> MAYIAVPAVVDSRSSEAIGLLESFGVDAGADANDVSYQDHDYVLDQLQYMLDGYEAGDVIDALVHKNWLHHSVYCLLPPKSQLLEYWKSNPSAIPDNVDRRLRKRLMLKKDLRKD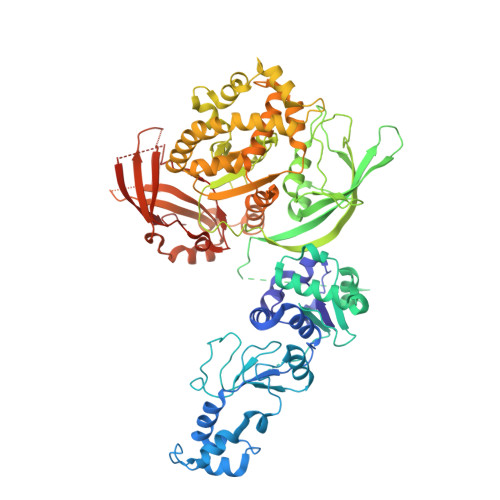DEYNQLARAFKISDVYAPLISSTTSPMTMIQNLNQGEIVYTTTDRVIGARILLYAPRKYYASTLSFTMTKCIIPFGKEVGRVPHSRFNVGTFPSIATPKCFVMSGVDIESIPNEFIKLFYQRVKSVHANILNDISPQIVSDMINRKRLRVHTPSDRRAAQLMHLPYHVKRGASHVDVYKVDVVDMLFEVVDVADGLRNVSRKLTMHTVPVCILEMLGIEIADYCIRQEDGMLTDWFLLLTMLSDGLTDRRTHCQYLINPSSVPPDVILNISITGFINRHTIDVMPDIYDFVKPIGAVLPKGSFKSTIMRVLDSISILGIQIMPRAHVVDSDEVGEQMEPTFEQAVMEIYKGIAGVDSLDDLIKWVLNSDLIPHDDRLGQLFQAFLPLAKDLLAPMARKFYDNSMSEGRLLTFAHADSELLNANYFGHLLRLKIPYITEVNLMIRKNREGGELFQLVLSYLYKMYATSAQPKWFGSLLRLLICPWLHMEKLIGEADPASTSAEIGWHIPREQLMQDGWCGCEDGFIPYVSIRAPRLVIEELMEKNWGQYHAQVIVTDQLVVGEPRRVSAKAVIKGNHLPVKLVSRFACFTLTAKYEMRLSCGHSTGRGAAYSARLAFRSDLA> MLRNTDVRLFSTFALNPETSVAPHGPPRGLVNRYVSMGLPPWAAWCNKVNRYSLYRMSGVTQRSFLPKPPQEMDVIWLNERVRERVRTSRQVQNVYRQLKYPYVKTGIHYSDVLDHWVQVPMVEAAMFEVEKDGGFDNFILKRSGPELRSTYGERIRRHILVRQKEIQKNFVLQKQAQMLVESMEKEILPMEDGKKVEEVLEKYGIDKEQLLRDIARAAVAKKQQLASAVPQPSHVEVSTN;> MQRNLTKLSAAAFYEFVDNNFLNNKRPPVPGGSWTVEVLRNKSLADLQHIWFLLLKERNMLKSMKEHYLRHQEELGAMPAPSRLKMIDESMRNIKRVVKERDEEATARAVEIFKERLKRGIYRYPPGPPPPPGAHDKTSVVKVELSCYVEEERLRELFGRYDVFEPHKGIVRVELKLPDEVLKQKEEAEQLWTQYMAECSDVKAYHQWSTAAPSAYDYTEVELAPGIFANDAISDKGGKHSGDTETHEGVIVAARVPVPPPKEKQPPPKNPLERLKAERRSYLARTTIQLGYFPNVTLPPPRYETVEAVPRPVHPDEIEGPWEAYITYDREDGLSYAQSLGITTIGVATVLGLTEHVREPQPYAVVDPVYCEALRRERAREETLMKWPHVPEWKYEYSTYTRKHLADIVQYNYTNVVDYVDREVLLTGKSVWECPIHIDHTCGGSKTVPPHAKKPVRYMDAGIANVGVTDI;> MMRRMWVPTFSAQQQHLHHAMVLKMSTYASTPSGNGVTSAASNEEMNLHDAAAIAPGPYRRVGNIFIVHCDDHPFKHSWEVNRMLRELRLEFKGQTTIVPDIPQVRKRIWRVRHIVKVDVLDLDEAKALIGVPEHISFTDLASQLPPSFGRVKAVPSPVIRSKMNFMKLRRMRLRDVLHRDALELRLLELKRSAMKNXEQQKHAQKDERTDNKEGEKC;> MFRRTFFTPMIAQPTLLMLGNKGGTPKRKKNPMQLRRKVYGLHFKEKYLKMEEWYYCPLCAEPKKPGEWCRREDCRQIKP;> MGSEESNNICAYKRTISLAKIYIVLLVKTAMLRYSRLCFPKMGCEEITRKARRVQLQPTEYLAQHRMQVWQLRFKEMGPPFSRVWVALGGKMRRRRVGRQVDVKDMRYYWRPIEPQYQRLYMSRLRIRDHSNKLRQPMRLRATNADIGSGSSSIEWERASNRKYGAMLAPPKRQDFEFRVV;> MRSLIAMRRRFVSGTWTIAVSTQQRHRSGSGPGDKRIRTDWYRCYPSLMREKDRDMYHCYYPYLFDHGDKMSLYPKIPENPREWQPEQLQTTYDAIREDKYDAFIRLREKFPELYQDTRAWDNPPPFGEFNMFYSVRFGMVGVKAFTCKDYDELGNQFDCTAFWFPDNQVVKHSTRNGEVGTDKVYVGAMNVPVEFHKPHVAAFYKAAGVPVKHVCAGFPITPDAYAPVGTKLDVRHFKPGQEVTITFQNTDYGFRGVMFRHGFDGGYVWLGDSRWQRRPGAMGTEGQKRIYPGHRMAGQTGAAAETYQGVPVWRIDYKNSLIYLPTLLDADVGTYVRFSDTINTKGLTLWNEHRGLPAFPTFIPPEDEDLSKLATDECQLKSPPLYMYFRDEFPATQLVSQADVEDAKSAKPATAPPKKKVYDMKKYYEARKKYRQSMQKARKYKLMGLRTKAHEKQEEARRAKILKYKRMK;> MRRVSFSVVLATFGKRHSSIFSPRYDWRTSGVHDIAPRDEGDFLYQGPQHVLPGAHPLPLHHPHNTITRPVISPYIPSPQRSHPYFTAPLPELPHFSTTKPIVYTYGTMKERIIAPVFNLKNEVIYTRELDPFIFGMYPEVEELSKNLTYWMVRCQNFASKWDYETREIWRKAKKNWPNTGMGMPRVGNRKNHLYTWGGRTKPSKPWNMLMPTMDVKTWSKSNRMMLTLKMLQGRLQVVDRLTLEEPTQECYLELCRNMSWDVRHTGGGVLFMDGGSRITPSSEFDRAFFFGSFFNGRNKIVRPTVLCDEQYDYNKTAAKQRMKGPKGAKNPIPINRFNAYDAMKHDRLVITEGALMQLEDELYEHKLQILPPHIRNQLPEYGYLDSEALGDCVPSLKTIQMEAAARTEEAESDMYKSFIDNPYNPWKDNMDASYAVDGADGTVQKFVDGKKVSWSMLS;> MRRTVVQRVAPWVPPPRHDIKVTMPPPPGGEVGGRFGVSQGYSDRLARTPYWKRMALSTYKLRMMENATRYPMSEHRPGEYDIRYLPTPYPCTIRNRPLLEVGEPRQIPSIRIPVIFLVNLFDEAKGCWFGRRYETVYVERQFMREELMPQRYAIYATPEAYKLLGLPVVNHHTHEEIPKTPREYEKLLERQRYDEERWKYTIEYLFRKYEDGPPELLDRPEDGWDGSEEIALSSVAGAGRDGVVSQRXXXXXXXXXXKIKLF;> MLRACGVLQLRARPKTVCVEPGSNRLPEALVVEKARDIFGRPEFPGKRVLHNWRFFIKAGKAATGPPVGQEFSKLGLKAMDFAKVFNDRTKPHFKEDVELIVRIQVYFDKSYLFTIEPPPTAWFILRALRKKRRETGPVPLRGHYCALMTLEMAYEIAKMKPLCWGRPEYPLLETRVRRVVGQARRMGVCFIGVDTPYSSPVKDMTEQQYTEECERYRRIHMEQYTTLRQRELEEAPLIERLHRPNMSPLTDEQIEEGLRDPCLLDTLWRASHPLSPYHRDLRERELARRYLNARGWVKDMTPEEMRIVFMNYRLPEGEKRKQMDEXAMSGEVYWTRDGAQL;> MQRSTRIVMAPFKSVLRRHKHHPEGLPLYNDMSKQWLCREGERWWLLDARGEQLPRVAAVAAQYITGQHRPDFTPGMITGDHVVIVNIKDVVMVGDQWIRVPITWQTAYPGGKYRIRLTDMYERDPCMLMWWFLKDEVNRHFVRKLKTRIAPLEKAWLYEDSIHPHADKNPRPLCWTDPEVKGWKYRDPQFIRRWKPNEFMH;> MLSVSPPLRRYRLFHPRREAIPMHMCPAKTIFPLINSNNLLVKTRNSWEDFTGRKEFDEDHPLPVVGSRLNGRTTQHKWNHWDQYLNPQITQSIKDLTPTPEYVGMRCGHNMIKMGWMKIGGSWKYSRGYNDRRRVFARGQWQERKMTPRFMLAPRVSAGGPRNRYEGKLVFSPLRLSKLLWAIDTGRINPNEVITLYHLRQANVVGEREIVWPGFVLISNGVRRVPYPIHIELQNASAESIRLIEEAGGSFTCVYMTHEGLYQELHPEEYPIFMDQELPERRGLESLATNPSKRGWLTRWYEDSSKYAHPAAGRRYSHYLKPPTERDFPATVEEYEMVKHHQKWHLNQPGTGTLLPWHSYNTADLVKRAAGRL;> MLRITLLVVGRAPPVIGCTRKARYAGIDDNPTITYKPWDTTEPLMADYGWTRGKLPKFRARSPFHRQQIARRMVTEMIRKDYCIVGGARAPALRILADHVVELAKAGDTDSRQQLAYFLHDPLMVDKAFDEYPRRFKDMNAKYAMMTRLKSRRRTDAVAMYFVEYKNRDMSDNHKGEDYSAGPERFFLPPRIVETEKGIQRPPHMQMAFDRWASKFKTEEFHHWWRLRHAKLRYWGVRNVPHPSDVDPLWTEKEEEEWHNEMLANTGEYEDLDLDDESYTAAGEGGEPSPAGDGPQPQRVG;> MGYTRERTNRHFFVARANAFFSRLPIARVQRSLAMEAVREGRMRPWKYTKEQILGAPVTCNFEYNPRPVRLIGTVMDAHTEETSIKGGLKVYARNEETNMMLWIPPGNPKLRHEVTSTKGSFQHYLDERDKWDEAWITGRARMK;> MLRRTVCVQHYRAKLELDRIRSMLRGRARLERKVGLKRLFFLMRTQTRYRVEQQAHWERAIVRKNVDSAAREHGTGWQHLRNELGRQNVMLLPRSQQLLAQYEPLAFRAVVELCASRIPPPPPPVVASVPEESYTLWPPASHDNSECASTDGSDAPHGQQQSLSHPAARVELRCGVERVLRRGPSGLGNNVNELIDAWKEFDVSPLRKGEVNK;> MPSLANGLRCPDALITRTLNPLLNGPKFAVIYCGNHQYKVAVGDVIAVQRLRVEIGSHIALKKVLMVGGPRFTAIGRPLLEGVRVTAQVEEQKRMRNVVSLFATPGRRHVRWVDAPHAATIIRICEIFYSPNVVGELDKYKGELLETFTPGQHTNPVYPVDDGYDVFRKKDKEAMENATTFLDLLGGV;> MPRPAPRFAMGHMLPHRSNVGSQFLHTQRHGSRSTWYKKHYFSLRPFAIQRHHGTTPRILLDRSLWKSLWITKLQLPDINRWERVVNSRRVTEDRYAFVEEEGVMHKVNWGLYCERLETELTVTQERLPQHTLLMKAVPSSWKKLDIDISVIRGLSLREAMAQCKLSLRKGHQIVFRALEMAQQGAEAKGLDKEHLRVAHISCYPGPTDKQIDIRSKGYYAWKTKKSSHLVLTLAEDPEMVLPDRTCLPYSSLMSMKRAGLSAQPTVIDVPAITADGI;> MVVSLRRFHSYANSSRGGATTCLITGGGKGHFALTVSTRGRFYRPLVDDGINLWRRRMGRIHKGWRTWEYQHTRPDPRPFPDPPVNDYFGRSRIWNPIACKLGYVRKKADEWGWPNKPPPPTGLRYSQEFFPFFFERYFPDAEVRLLLDSVLNNETKRPVFQIPCSMSKVELVNYLKNIYGIDNVVRVEVRNRRGRRYKNEVGEIKMMDDYKVAVVELDTPVSVELKQIKGTEDTSDNRPQERITQ;> MYARFRTRSKFYFRPARPALAYNVDPNVMRRPKVKRGLLKGTYSDETVDLRDRERLELLESMRHPRERDFYQDHTYHNQWLRRDLEKHQKQQLAARYKYFAPDFEISPWIWYPGDIVEVVSGEGIGQRGTIIAVIKYKNEIVVQNINVQDVVIPASESRPEQIVQREHPISVTRVRHVDPSTNEICNIEMVKVRNKETGEMEEKRMSLESGILMSIPPVNDELEVGDPLKDTPIQDADEATYDREAEQAVLVDKRLEAMEEHFVQSLKQSYEFHEPLRRKNAEDMRQFQTDVIDMACAMLGERLLDTVNASDTSSFPAEWQEAIAMHVEEIEAEMEEVAAKEMAEAKEGGAAENEQHDDDLDDDEDELDTSEESVKHV;> MLRCSCARRRGVYHNAPSVYPFVKPFHDTPYDQDRGRHDSVGQRYRKNSWPEWMDNGADGTGYGIGLHRTHPLSRLRGNLKRSPSHVPRVLGMMIQGVWHKSGVKLYFRGGKPPNPSVHPYLTGEPCPLYGWKVTDESVIRQFNMPSIDGTNFRYKPYVALQERKIMGVQVPSDSVSLASGRTTESKPLAKRLFFWR;> MLRLCRVSLRVQSHQKKRAQHPNAGTRFGRVYNRGFIRYGFGGFGMSVYTPKKDRRFRVQPLPSLHANSLADDTPLVTTTRTLSPNFRAFALQDGGVFFTHPSHEQVMRVGQNILAEETKATGMTSMDTYVNSRIQSIIAENTVENVALSHWRRRHMWNLVRTHGKLQRHWGVSDATKGARSNIYGRPS;> MSRNGELCLKKVIISYCPSNGAPNTRQFLATHLPHFHAKYPSVSIDLRPRLWPEMAITGVYRDGSERSYNTKNLSPMGIFLRLNNLVSTANDYDQPFCASHLHFQRRSVQGTWNPWLWNYETERRRTEAPQWRRKLSEKEWDYYVGQYSAQMKQEEDEIQRRVADRTCVQEQSTREVQERWKRHVVPRMQTDLEFNLSHFKRQHARGQLQQRPVTMGEYRLFSVPDPRELGQDAVDTMRRRESHNMEVWWRKRKEQLKPP;> MLNRSRLRRVWLGGTAANTSLGRDVMPSTGKYINIVSPTDVAANISAGAMPPEANVAAALPVPRIQYSKWNRALRSDVYDELLKLPLRYKLHDFAKLCPPQRCQEEPEAVGVVGRDSAVGYLPPLGPADPLDTIPFFVHRSSNGVLPGKVFSMHPRNLMPAFYLRIQQVEGDMFRFEEELLKIFPTKKIFVRSHSIYVYNVALDGRMVLHHWLLGLGF;> MHIWRTAASNWVKRHARSNAAQWRRPEPASSSAAAKTIARLLAVGGHGCWSEATALYAEALATKSVQRYGVVTPAHRHDCIALILGAMSSSVDASGSDINRGEASLTPHYGMLAERLSLDIIVPHSDVGQEEKEAASVACIAVFRALLTSGRTHAAQRFAQQLLRSRNSREHGLWALRTIMLAVTAREEGMYRQLFLHGGLLKDLEHLTGLDAFTVVMSSCDGHEKNIGPCGGRTEGNLGRDEVHRVAARWCVDVALHMHTCPWRFCLTNEKEPRRETAFNSEVTSYCCAKELPMPAFAVTMLPFEVLRSNAVGVLRCCTAAGNGSHGNEVVTFDGTASNVSGGRSGDSTSCSTTAPSLGLPALKRLQDVVSAAIEVPLSTHEPVECLYLLLQISRDSTAPDPRRVMPSTMNILWWRRHLQSCVLESVKSAVRWKSVCDFVGLSRLVTERVPHCFPLLVAHAAESPDALRTLFNEVSRQEGAAAXPVDDIPRSCVMGLLQMCGDERSAAVIDWVVEHCXDHESIAQFVLDSLGQHQELASVVVRRLFQRSEQSXDVINALSRLLEKGTCRTLLADVCSLVPQAQQWTVALRFVSGMSAPEVGHVHTAFMAFVGNCDEQFAINMALLWSDETFTWLKADVNPPPRRVYMDDRWSDALRLVALGAERLTQRPELLGKYIRYFSKRVAVNSRLYMELEALLACSKVGGGSARNCGRSSNWNPIASTVTGGPPLETSLVGVRTEVLPKGRQWMEACAHASEVGVTRGVLEILAKRGRWEEATILLARAEAKRRVEWAPLVIRAARLSSQWRAALSVAEKIAANGMKLHYSVVAELLACCFSADVPLEVVQLWLHRRSVGESTSSHVLFGLGPGSSLRTEQRDANDKHNVFGDASRWLGSAQAELFFVLLESSSSRSSDHQWRYALQLLKEHVLLSGGVPSARVFRSTYSILHRAERWRESLQLLGLQRSVCGSPTVKCVHLVLSTLPSTAWQYALGALQCIPPGDSGSIHRVLPLLLPVSWESALGLMIDHRVMTNTAMECVVGCEDVPLALRLQAWRRLLPSLPVSMKHRAAPIYLRLAAGVADGDVGLEGTNGLDAMCVIERSIRGLRGDYINYASFVYHRALLHRHWCNDSLHPSGGVAAFRALSGIAEVDQQCEVSAAALEQLSNIVERLEQVCGTVSASTATHGSQHLERTVPVVNSGEILQGSAPTNARRDPETHCFSFVSSYWLSLFYLFRYCRCVISSSLFPFFKKDQGSGLPIFDVMRLHTVRAPIITRAAMRGYSEARSNYDGTSLPAWPAPGKKPTYPAALSELRLPQPRMRKTRTEWMYYHGHGGCPGKYGPSREIADFEYADGTPASISGRRFAFKHHQDHLLVQLIRAAATVERYDASGLLPRIPGTAEQRNWDPAIPLFLDDVDEQGRPAPLRTAGDAPGTMVSHVCSRVVDERMGTPTHTPNELANRHEGETLEANTMFATNDPSAFVSDTVKLRDDKRPYWSRRRWALTDKFLVPKSPKPKNTIKDE;> MLNPPKHYSVESLRTVGLLPAQLALSRKPRLRPHVGNLKGLVYPLPYYAMWRGNHNKYTYNKSTVCLWGEGDTRSMYHQHYAHAKCPTDYGRGGREFEYLTVKRGKMLQKPLPRVQYVAEGSKPVWLFKSWHTPLSSPSMWEREVQYAEHTPEHIGAKRPLAVVAPRTMHRYLFLMHMEKVTITVSPLLFGYGHTIQKAVLDFYRRAISARSPFPKDKVFLFYAIDHITPRIEVTWLDGTSYVPPVLEGASSQDLIQMVMEEAWLAADRMAAEGRVLNPLAIDDYKWDQLVVFKKVRDKEASKGGGRKK;> MLRHCTAHRRYRTAWRELLHPLPVRARKMEWLKRDAVEENEEILRRPYYTIKSYALPPAVGRQESIHNSNNIRGGMHSSHSLDLIMRQPRRVKTPEQLRALRDRLRFIGVTGPMPQATSVSTKSYTDTYGSRLRPRYPESWDTVPPHQPSRELL;> MLRGTRGFLAVSPGVGIAPETTPVKYTPMMLNIQNMMWWNGKRNLYRATYREKTWYEISRTGAFTKGRRPVMRQKYSREALQAALAMVPPGFEVADVPRPPQRILAQSEGIVGRWYSNYWTLHSMRYQCLLAGVEWPLGERQRPRTNYDEPFFFADFEESKAIRDYRSRWINVNRSLVGMTKRMKEAEEEARYMQFRKLQDTFWSNRKVLVNRVKSMYNQGARTSAKDMPIKTINIKAFLSE;> MLRRFALTSSVALRLRFERDSGHNTVRYRPIPESMQPKHLEDNFTPFPLPKFDESLEYGPVRLRNIPDIEAAKERRRGSRLAATEVLLQETLQEENQFATSGKGDGNMAIAITERHTEDVTTPAADSRFPSQTMSPCSHEEEMRGYVVSRDYPLIDRLHCTRSIEELVAQFEDRPQIESRVAALADMASTVSFRSDEELLRMFTAISAPFSVDGRGLNFLTVKVSKFGRPYYVPNSLLPAYVNLVDATTIALVREQPWRLSASPALFIQVLQFMALIKVFEPNKWFTFSDHAPSNRADYRHAIGVNHSTAFWGTGEELYDFMVELLRVEDDGRIPTMLDLCTREQMVDLLSGFCGVMPCGKAVGDVFKTITDAFLRRVRNDISGPWSAHDWAIVERMYLVTVLCDAGNNEILQLLLSDTASPRGPDFFAAVSRTKDTPTKKRALCLLQEAIDNASAKADKVTLLGLLESGSEFLLSLVDKGVAHTFATQNLFDYRILNSFLHCSLVADRLRVEQSVITSLIPSSLRDVQVQMLMSNERNALNPLTSSLPGNSGAIATAPKLKRPLMTMLSQLEYLNSIDSVFILHSSLMATSTDQLVSAVRRLPSGKDSLIVTMSCLRALSVKSLTSPSMKERIACARALEIVSYELEKGRAVLLPFSEEILLHDAGAYCDEDLMLWTVAAFLARELPLVKVHTLMHSNCTARTPYRFLKGGHNLLVSSRSLYDKGAPLLSSLHSKELRLVTHNVRLRTPVRDRKCTLQYYNPIRARFVYRRDKPLFDKYHVTARNLAPGFSRGALKHDWRALGVYTPDHPQVPYHPLQTWMLGETTVEAE;> MLYTRRLMTTGGSATADGAVSYSKGSYHIVPKKYTVGKRIAVRSYLDRNRTELSDRTYMPQKAWFEPYTPKKFDMEHQRISHNFYNLETKLIWTAFDTPELIGILLHDETIKGAPHLYDAEFLESAVHWTRESRYWRCIGITKPFYNKTTLRAQCWHDRGLQVGTLVFSQAMRDALMDLERAVRRKELGLEPNYVWDRWGPVGFIDGARTDHLPRFAHNPYVDPDGVEVTEVDIAPFNTHEQIKERYGAFIDPDLRPFEGVFRAPSHGALTLDDVPHQEAVRLYRDLMEKADMPVMLGNGAEIPPMDMRALFHLSANPERMKAASELSSWREVRGMLAPVQEVCDEKVEALRLMENTRHDAARVRTFYEEKCGFSDFMRTPDKVITAAVLCYLQELQRICTETDWGKPLARCLTDLERVNVMGKDAFLVYRHIEDAILDKKRRVWATRFAGEANEESTLDYLLENFGRRTEQTRNVGTTGTEFDREQEPIGRQVQRRVLDSDKASKLAEVRQKRGKMWSNKKSVFDSLHQKQLQNVTYGVH;> MCLKRKAPHLFCFCLWSIFLSFRCFCFRSYAIMLPLLSFPTIQISIFLSFKLPITTFLLSPCFVFVFVFAIRYCGELTLNAQLVLFLLYHCAQTQRGPLKEGEMPICPGLCGELAAVPFRVFLGTLPTLAVEERFLRQLQPVFAWYSSRKRVKEQANEFIEIDLASCDAELLLRYSHIYYVRRQLFDELIERQMTLLDSGKAPKMAEPSLLQCLAGCNMTIADRLQLEIRQLGAAKRAASVPGRRELDPVARLEVYDYACMMRLVEEDAGAVGDAEMKARAYLPREVIESKLGHLTQLLLGSDARAALDKKDVKLLNRMIPPDYTRVGCVEKLRPFDVTAYFRFYGERINNVKVENYFKRALWGHVYRRFATTPSFLSGVSTYWARHSGLDASFTTTTMPQEVAVAVCDQQIQFPAIKFRAQYVYTSPETARQLWRTDAAVPLMRLFPLMGSRTAEDLAAGVLTDAFWMHLGLSEEENLLQDSLLLKVRRFVDEVGDMYETNIDSVLKRVDDNFKQVVPQLKAEDLQVDAPLQDGEGEDTVRETVAA;> MLFRSVSCKNYQRGGWSPGSKHQKHMTLNPTLYLYRFPGPHGPGPYTMKYWWTLGCFPTGMEVPFRLHEFLSTYQQEHVPVEVEEWLRCYIKDPLSELVNASNDFFKAVEVYPEVESARGYKTLQPSIAPLLVPMKKFEEQLGVKISPVGLRSVLSNPVLKDRFLDDLFDYKSYVEKGGSTPHRRLARSRFEGSLSVLGECEKCLPEQHQVEISESLGTFIGATVSPAETTADDERSLILLLTTISEGCINAGNYSDAASVLADALMFCHDPDSQATTHANISFASLLNADFKGAEYNGREAALLQPQVKPTSTACARGYVGWAAAAAYQDDFEKAEAIVKDGLTLYVGNEHLEKLANKLQALREEQPSVYKQVPRSLRESRSHLPSQQSRGLLSGSGKGFSNEFDWVEFKNKLYPSKMDPRNNEMGSVFRRVGDLGSFISTSRSMERL;> MSRSAFSSRGALLFSSAPLQCQRRWVTRLYTSYYTGVLYPNQLVQPKQRLPADVSVSAILQKRSEPEAAAERGSNKGDKVDVSKGEKTPRVSWDDADSTDVMRVDNTQQLKEAPQVERPYVPLGEVAKLELQGDYYMEGGMFQEALEHYGVVAKAYNYAYPENHAQRIGIRIKLSAAFRQTGRLESSLANIEEVLRMLDASTRPSLELICEALLELGITREALGMKREATEAYEEALEVVNSFHNWGESHRMLRLLPRLGRRFNYNFEEKFVYFSPFDYDRTFALVDQCLERAETIFNEIGDVEGAIRVLQQRKEMIDKKFFNMRDFAGRIHTMRGHWKRRAQHLTNAPTPDELLRYSPTIHQVHRDFKYELTAPIGREKEVMPGVNRLVLDMGNPYRRRGRLSNKMLKDADHKFANYVRQKEYNE;> MLVPGLSLTRRAVTSSCCRPLHVVRGFSTTCTLFGLEQLQDVPTSTSRRPTGLHRGPGKRQTSEREAAQYKFIRRWELQMRDEWDQLEPFKGLPKPKRQFGNEAAEVIWPYALLLERVVKVHPFTKSIYVYYAQRQSTARGKLAAEIARSFAREFLIPITFHNSQVYTEAEMLLEYSETPWVVLHSLDNGQKPRILPVAPVEGTPAHTAVEQLLAEVVQGCEALGASVADPVTATRVLNERPLQNQYVRVDYQWFGDTPDERASHLVRWEFEPEQIEPKIRHRTRHVLDWLNYDGNLPTHRAVHVNAMREKARQKAPRTVAGPRTFYNSAGSRANARSSRFGGQAAVGK;> MLRRSDLLLKKGWTHNPGRTRRGGKNLAWRPKMSERTLEQFVPLHLAFPRRHPNSWQERQFHLLGYVKWPKEIGFYNAGDNFELTPQAAYRIYKQNCDETFWTRLHNEKTIIHLLPLVEQDPGTNMVLVDDIFRHHLKRFGADHYIYNAVMQAAAFAKDFPRCEQLLAEMRGLGLEPNAQSYVNMMLGARLTGKPRDQAEAFFREGIKTGAISAVMRLDTEFQMWMNQLERLGSFKAKVGYLSVNEEGASPMPRDMWALWGWHRTEAKFISRKQMISEQVQNRVRSGKELVGTVYQKARRQPWAKYNGMFPYDYNGPARRPAASFVDAPTPTHNAEVCGTAY;> MLRLSSWNLKSQHHNVLRRSRPHIHKYRELNRWQRQAQGISKWDQSHSHRPLPYVERFNPESVGLTRGTSAFAWKWWHTQYPWLPNVPPEAAQIDEAQKQERRSHRPPAWDDEFAKVVLNMNDAEIREYLMSKLTDVIFLETQRDGYELRRLDFEGKPLTSLPEPRIIENFVLEEETIRERVIYQVVEGVFRLSPTSADRRELRSVANIIDYVLTHVRAARPTDRERRQERPITSAALAVMQKCPIQPQLGFVHALPHDTRDALLQEWERMHHLDWQFGKAVYTPRSKENVRGNLTWLREDRHYDQRMKFMQEVESGEARAKHMKLIAEAAGN;> MYVFRFHISSFHSFLVNFLQPSRGVGEPSRLLXHLETHPSYMRRVTSTAVHRTVSSVLSXALLPSFNGTLLLSVCFASCSAAPVRNLYKRLGLDHKATSEEVKAAYRQRALECHPDVVDDNQKAQAEVDFRAVSEAYDVLIDPQKRKEHDKALGLERTVPPAKKQQEGEGVGCDSKGSFNRGVTRPRNRKPFVRGDADRNFREAFHGMSLDQVLFRERLRQRRMQKQMEEKAKEGDDGSPAGREESIRRVAAAAAERFAEKVRRQYGPGMLRHARVYTSLSRDPQPPPSDYMPFRPFHGWTVPNGVRTPPEPTLGPTAKVEDVKDVQLAEPAVGDASHQRKLPKHFPVVQASDGSSLLREETIACMERERRLPHNMGKLYSYHRPY;> MGASAGLIRRGGGVFPDAVSLTLTPSRRVYGGSGRGDLLYENPDARRHSGRALGVLNGVRHSSQATMPESGQLYYRKLILHSRPPNGSCAGLQRHCHDTCNWSYLIPSLHRCAESAISAKLWEKMCQLGLEDRSKAWVNLTQYERQRVRDGQNLYRYEVHQRLPLLEESIGWAQLDDLLGWFRSARRAWVRLPTSVTLSRESSEAGVASVVSPSSAMSCRLEGHADSRDTTPGRNQVFDTPERVEQLTEATVHRIREELQRLNRSERSDCEGSAAMRASARRLARDEELSRCVEEELGWHGVALQHRIPVPK;> MCCLYTSDVFFWSSLVVSPLPRIVRCVSAPQIRSIPCGSGDFSVMKRSLIARWQSGVHTPHGVVYRGAKMKNWPEQRIPENFKFTEEQRFRTKAIPRDVGTIPRNFVLGVLYRHQPCEVGGLWEHCTNDPEIVLDSKRHLREVLKQAREEGFVTFERDAISNEWLCFLTRERYEEVQRIVTAKSEAVDTHSGLRGAAATETSTYAEKFREMNVEAKEAHARRLEEEVANTTRYLRRFQQREIDYLPYTDLNGKVNFMWWYETRDVQQRADEVLTDSSSSKALAGEEEHKAGSQLEATTASTS;> MKRLFPSAGVSVVLTSSSIVMSCPCNHIFTSRRAYYWPYNEDFVPEGAETSRFQSSGSPGTRRRVLQEYALSPLFGARVPCCVVGTLRTAKEIIVLKRDIQSLLCELMELPQGSVTLGPLQQLREMMLYRHGTPLSPRLGDERQLNMDAYARRPIAARTMMDVFLAEDMSLDEIVNFGRLSLGKLQIALNNLRKENAEKSSADCEDGSAVEPAQLLVDRMGISYCEIPSLDESDYVFAEVGGVAVTDEEAERVAQRWAERCE;> MLHRTRLAQLINGRILQYFVPYERDEVNPVVFMDVTVEGDALGRVSVELFHDIVPKTTENFRSLCTGERGYSQCPLFYKGIPFHRVIPGFIVQGGDILLKDGRGNVSVFGFPFPDESFEGKAGKHLRGTVAMAHSAPNQNGSQFFFNLARNDHLDGKFVVCGQVIDGWEVVDRVAVLSGSSCGTPVSRAWITECGQSSGDKLEDTERALSGERALHTMPGKEVLDILSPRY;> MLRFTRLFREMAPELQLEYMPVLFTRTILGPQGGFAGEERLVKLEVARKYMEAGHAVTPTEELRRGLWCYNPDTDKYDCFIERNEEFLDFAARKRQWLDVYWRVNTGYLLFGRQSWGQGFLINCPLRKRDVAQKLWEQYKVRIDPRLIEFREKDRRTGIQELGHNWCWLYLPGAEELGINREVYDNKRVKVRIHVRKMNSMFALY;> MRRLGVFCRGQRNSPLLTRGIATGGRVTNEDRRWWLVHLECAPDITPGTFIAWLDCCGTHTCKKLIERNIWTIEQVAALDSDQVDELKYREGCLKMDVVWEHARTIITPLRQREVTGGVESELQGRIMELRKKRELERRREEILKERANVSEQREETLRKLREAIAAKKAAMXQKKQAASEAYGGSSDGGARKEGAEE;> MRRCIPARGGFTMKYKKGTGLWDEDHVNDYKTNRYLSARATMRWYQEMERHQTRNSLNARRATQSHNNNRGLHHTGRGAFERELERRGVQVEKYPLTTTTGTMRVAELVILRRMELEKRAEEALAEQRGELQKKNPTPSEWYDESKGPLNPNFLRSMRSHYEVDIANLPDTPLIRGQREFFIGEERGNGAA;> MLNPTFSLYRKTLQSYPVPPKIRHYDRRWSGSRTNPYNRQYWRVIMNENYSRPSFWVSDFRHRYLMRTGTDYQGQVPSSPQPGLYQGFSDVHKLLANHPKPQRESRHLPVLPMTPRIVFEHANEKRIDTAKRMRRDRRRIEELKTLEFWGWYMKLQRVRGRWCREQGVSSRGVYGPAVDAAELWG;> MLQINAFKLVRATPFLLKRTGKPADTPDYKQVYLPYDAAPTERELERERRRFKQAYHGRMEHRKLVEVKEVPLNVYTYGKEGMSLPIAIFKDQKDPVIGPEWTYPGIYENKIAAQHWYTEELFDKESKEAFESPWQQQILDNQVKRRMAKVMFRMRQVNMKAVDLFQKERGSSRRSGGAGEKGKDGGGKK;> MSGAFGCGSYRSVVAGTQNVPRRMTFYPSAYELIQLHKAHREVIRHFYVRDKIFDNKFPGNALANGLFKFVPNRRENYHMRELMESIRRRSIWMHRIKQQREINAKVVENMEVKYGKKAAASMLCFTTPDSNAYFAPHRYQDVANSWPNYWQHPSVNHVVPKPRWRRHRELGGITRVEDPFAVQASDY;> MRISERAFMDIAIGTKAPRRIVFKLFPRKCPSAVKNFIELCSGNVSTDTYESGNRDKLISESALPQLTYKNSTFHRVEKGYLIQGGDIVTGRGTEQLSIYGGTFSAPEEVRASVFDKPGLVGTASSSPNAHGSQFFILTAKEANHLNGTCICFGQVADGLDVVQEIEQVPIDPSGFPSLKVSIVDCGVLE;> MFRVTGLQLKNPVVFKQGQGMFSHQLKRLLQKKSIHRYNWDPLPMYDPRKLVHASRHMDVETWREVPDPHWDERSYLVPDQMFYNIPVPPEYKDAYWWRELQARRVQCPVEWVSHRMYNKGDRQRYDFQDLAFRKKFEFSYEEVVKNAKDMRS;> MAQWVPKTAWKVSNLNKRYGPGYITSGFSSENTLGYTHMVHDSHKLREKLSSRKGIFVIDVRDPGERKLNPVPRSVALHHHDLLSGASCPILPQQKSAAELFVLASNESRGLNSAAALRRWGYDSVVQVDYNTLVEAGYVSRCDYATAGTKDSAEQAVSGED;> MFRPTTAIADSFKEHYHRVHLPRRLALQRYARQQSLRNAAKGNVKAEEVPYKYNRWWVNEEHEFVHQYAFVEDPEVTKAKRETLPPVTRENIWKEPQQTFFLPFAPYVRVVDYPKDPDAKFLKPVNIPRWKDYMQRTKPVIPRTWY;> MVLRGVRLRSVAVSCYGSSLTAATRCLSVRTEDFFSKEAISHARRVSWAPHTTEKKQGAFAKLARSNFGDPLPSSFAQEPYFEEEIEAHRKHHRPDVYIYKYNVSPTHFSLRE;> MWHSSLRYVSFKRLPFGRRSTSGGVNFNKGLLTDRERGDPFTEPHAYRNKKSIAAISKVAKKQDILLREEKQRKELDKIQSGYVTERELHIGCDKPLGGNANEIARVIDEQALISPTPGEKCSTALRELMENEVDRRNHMMDKFGQPVGAREFHRLFKELRHADNEAETIERHQTRLVEEYGVYPSLRLDAYMLDDDTYFPEWVNALPYSIRDRVKFGSLGLTEKDEALRVTLGRMPLDRRRREWERLKKAKEYKAAKEETLTLAELRDARQGKRRFHWLQRKRQKRASILRRLALRKPDAFELWPSRVVDYSQRIAFIAQHVENGLDTKGQWPLDPEELARARVRRSKEEAERTFLMSAEEKRAHKKLSGRSGDGSISEMLQSLEVPDKPFKRLSRKVYANRVNAIVHGDQDEYGRRYRKMETRSKRRMRPYASLGEIGLENELRKEPRINAKGLNNTDDEDWPRHTKSWGDGMPSMRYGS;> MYVKLQTRSIPSLFLPCHINFDCVVCGGEGEQAQGKKDTDAHILVVCVLQQYSVVTNSRRGNRSSCSRIMLRSFRSNAFGLLIPGACTIRGRHLPVSSLEVTVGFTRLTSARALFSATHLLWRRQHGPTNVLFQLDALPPNLQREFHKDENAVNLTYLVDLPSSKIASSHEDSSDGTTKSDTKSPVIKVLPTWAHIVTWCCATCGCQWSARPVDRTDPQVAAFYSCPRCAARTAKTYCSDTPLAVSPSTPSFPPGRRFAEAFPLLAAQWDACRNSVIHNKVLFESVADVPLPCATIAWWSCPHCGEPWRESVNSRVQRLVQQQQKHSSNGNVRSNNTCIPLCPSCEDRGLSLTVPKDGNEGSKEKSSSERRSKKKGNQNSELKRFLKDSPLLLAEAQLQPHEDPGTIALRSNKLVCWKCRRCTYEFVASVADRFLRYKRCPQCTGEKRTPLNLLSIQRPDVLREIARTVVRGKLLKMTVHDDTVVPFVCRSCLSIYRMPIRLRCLLPEGTTACSKCMWSRSKFTREVVSVGKGQKGAPFRSPPKKKRGRDSYAVVDNELHLRDTDLMN;> MMHLSLQLCKPKTLAHMFRKLKLAGAHPDVLWAVDAQKAQHNSEEMIRLETMMHQRSTPGASNNRQSTAESFTFWLTDNQQQPRAFAAGRSSLRSVSCTINPIAPTRTIKQQLTQLFRDAGVYEDFEIGGEGVEMNLESVLLQADERQEEHLQQSGTLYIRGDKSIEMLRRFGVLLIIEEEGVTYLVTLPDVLDKPVDDTPSTYTPARSLIGPDGEIDPRVQDYIRDRGLRAFDLRMAGSHSSVERFVSAFERLERLYEVHRGRAMRSCVCLVLSIKAPKCYVAEDGCIVLSVQQMPMWEEFLLSLPQEVWQSCVQMHRDWRVGNAPKFHEQQRQLMKVADMFHFFRVRLDGCIGSQTDWQQQFILSMQKEEMIVRNAVKKYNLKSELLKRRGEICVSNTLRSAVDPTKEIGYRIGGDGRVYFNHSAMNTGQMLRALKDNLRRLETFQKQHDDAVATLEHMSRSIPVDFSVDTNWKLREEGNLVSCLQRFVRTIKANQTQLSAFLTMLLKKRDGAGAPKKRMVWIISERFDTLPSGVVYIPWDVDFDSIKKHLLPSG;> MWSKVFTPLLTHRLTPAEKFPQLQLRVGQQRRVTCGRQLSIPLSSFDSHSLDFARREIEPGSVVELRDADHRKLLALAFYEPALLRVDIFHHTPKVVTDLPRISEDFFVNRVKEAWGRRQSVFRHVRTGSTNAYRVVNGYADGVPSLYVDLFSSSFARVVATSAGAERIVPAVTELLRQHGVEEVLLDTPHLKDHEKLTLITPTITLPETYMENGASNMWLPRDEYPTTSSNRWLINTAHRRIRAVLRDLCHGKRVLCVNDRGGAAALQAVMTAKSVVFAESDESLLNRVRENLVANHASAVFNTCETTNSPIEELSMRQQDVVFLEHRFDTLSSPEQWQNLLKVMLFRGVCGKGSIVVVAQEVALLGMHDYVASGGGVAASVVRATRSEMFNVFNRVTAEHGLRARLLRFFGPSIDYPTLPAVEAGCYSYAFLLELAS;> MRPLRCSFGRRHRVTSAAFGVSQFPSSSSTFSASCRWVVIPPVEPITSASASASSSSSSSRKGECRTSYRFAVKDEERGLYDHGVTPDARTLAAEAEAQYRASSEFLHAPAGGLPAPELHMEVDGTSVSCIAAPFGEEYVPSSKERFAHRGHVGDLSRQRTSDRKYLLDARSHLNIRKERQLSELLSAPMPLLQKSNEIQQMLLSDFYPQNLVVSSRNVEAVIALWAQCSLEQCIAGLNSQRPENLLAPSADTTCHEVDAVDSVPFLNHMKRLYFHSRQTHVAPTPLVLEYVMTALGNVTTADSRVFHLANRLLLDADKYVILPTRTTYAAFFTICSLHNAMPFALSRFKDAVVNLHVAVDSTMASAILEGLVQNGLVEEAVLLLARLQHVPMDVQLLNTALEVLLLSKQPQSCFSAFEAVRHSGVEPTADTYTLLLLACERSGLWGNTTAILADMQMRRVKGDGRTLNLLLKGLLTERLHGYSRQLYETMVNKNVEVWPALESHMKSRTAGGEQLKRGSTIKTSKSSQPS;> MKRFIQSRRVWNLMDIRRRPPVLNRLRGVLQFAQQPGALSRHRQGGDYNCSMRVSIYSRPGKVSRLNNADATWHNRSRKEKPPDFDPSAFRRRYRDS;> MEKRARLLLGVRMNYAPFSFMRRRRITAAALPVAERSDPLSICYRCVHERPFVEPPPEGDNNSDGEAYETARDALLQLNMMVRRGIEPDALMYTSLIATMGRARLEWQAYKLFSRMLESGIRPLPETYVALHDATSPRRHHLRCDLQQKIEESLETFPEELAEAELQLQRERDRLCVQKFEEYMSGVLPPAPPPPPSEQEAISVRDKKREGDRSSSFGGGSNAAGLGKSDAKPIATMHIRNPTDAWSTAQMMDEQQKLGNQRAQGSTAISLCEQLDKLHEEELRIFLSAQRQLRHGNKTDLVKRVLHCVSEKSIRDMLERRKHYFQSVAHILENDLNSLRRDGIIAENKADESVNNEGTDAIPSAANSGGSQPVIISYACGVDQTITAEEKESVAPDFLHTPWGILRKPVRHTSTGEKSRSIDRLQRLSLNVDELQLVRSKASTGDLDELPESLLRRYAYQFSLTWKRRHPLSLLEAVQWHSTTLLPQQLNEEGGASPTPALRRQQEDEGVHKTLENYEAFRIISQRTNNLQVVDNKEINLHLKAIRREALRKERRAEETLRREHSLLEAAALAASAKSFTPPEEDMVPSSRVLGVDAEHNNDNESSGRLLPTSSDWEKGESQEDEPKEXPPWAIFNGEEEFNMTTGRFGDPRIGRYQELSDGRFKILPSREAQSRWTVNRQLLPGALQDTLQRAELQQKTRVEAVEKVHQEKLKFKRYRKWDAFLRKAQDKQKGKPQTDDKEGDGDGKKSAGPLPAKKRLSLLLRKGKDKAPIDDAVKAKYCKTL;> MPRHLSSSLLQKSLTPGAARLLPQNLIPQRRPAPGRMTYRGPLLAELDRVRDTCTTEATSSGVVEESMVSNGAFDAVRPAALGSTSSVADEYLVPTPRATKLKKAAMAASRTPTFVLPNSRSATDGEGGARQANDERDGTNSSPQLFSIESYETQQRALRNIFNEAGRHCVRLRKDSKWLLEERRAFRQSHQRAPTTKEVSPHVDVALAPVGALKLSKYLSPCSASREVVEHSLLLHRTVTKSKLVQSSEKTLFRCLRCFHVYAARPRTLLRGEVAQSWLEYEAEAEKEERARQLARRPHLRKKKYSIGRQRASLANDPRCCPLCRSTKAQWMMEYVHHHTHG;> MRRCIPASVLRXVLLLQTRLVSTNTQTPPSGCATKIQNESPMNGSFNLPRERQILGGLHADWRTQMKRSGSILNDITPALPDTKRTEEQRRRVAGWRPVVKLLGDQRLRIAIVGRMNSGKSSLFNLLRLEPTVPGRSNVVRDFDGITRDSVEGQAQLEGMHFTIIDTPGMVQGRMVEEAFRTVETADAAIFVTAVDEDIMPEELSLMQYLHLKHMPVVLLANKMDLIQEEEEEAVLDRYNSLGFGNAIPFSARRKSGLEMLAAVLEPLYHIHAMHKVENDWDIEDLAMQGDESAMEEIRERNCSDRFIRIAIVGRTNSGKSSLVNRLVGFERNRAVDEKNSTRDPVELPCSYKGRKLKLIDTAGLARHRYRADRDFIGRIHGLSVNEIRFAHVVIVVFDATEGHPNKYDMAVLHSVAAEGRPFLLCANKWDAVLDQSATAEAIDFKIKRQVREVKYSNAVVVSAHTGLNLTLLMDQALELYDKWNKRVRRAELTRLWRKMEKSVIIPYHVARIGRITQVNTRPPTFLLQLQTKNDSNTLPKALQEMMKNTLVEEFDFRGVPIRLIQEVKDSNPDYI;> MGRRNIVLLHPTAHWTRARRSFVRSVALTTLLNCSGALLTTSRGIIVPQQLKAYGGTFSRSVGERSNHLVSDVVLQSLSPSSTHNSPLLSKNIKTKTVTSFEDMPLYPELRSALRQLRITTPSPIQQSAVEVIMQRKDTVVAAPHGEGKTLAYLLPLYQNMIKDRDVYKIPLRERRPRMILLAPTRELIAQLHHVCSVLGEATGLHAISFTSRKRANHRLSRLLKQQLVDVMIMDPKIVLRLIRARRVFLDDLRYVAVDEADGMLSSQHDHDAVHLLMKVQKRVMFKHLWPVQTQTVFATAFITRKLEFVVGKKYPDAVTCIRRQRMHRPPGTLRHRFLPVEREREKMDTLQHLLKKHGNRPREILTDIEEEQAYSKPHYLSGSLEELVELRGLHLRRRPRMERHDHEGETPIATLSSTSAGDVSNYKVEENRSGFAAKGDNADEMKERVRHALEGVRPVHWEHLTTVAAPFTCHVPRTVFADGKRCIIFTRGIDCATAVYHRLRGCGYTCSLLHAALPAAVRRRMFADFASGRTNILCSTDVAARGLDLHVDFVVNFDMPTNALTYLSRAGRTARQGRLGQVYSLYTKRQGVIVSAVRAFLQKQLPLEGISNWKRHMMEPRYAEWRTHKLNAIARSYVSLITQKTIPAHLERTYLRHNATWRPLFHPQTTGVHGGVPPRQQQRVMDAITWKAVCFRRGLLARRKGGRAKFGTRAAESGVWNDVGGITSRVVANMEQNPHPGGDDFGPPRGPPK;> MLHAVRLLSCWRPAAIQHLPDVAPXAPVQEVEKSHARYRPLSLRARQTLSEKSDDLQYHVVTQEWFGERVDSFLTCHYPQWDYETIKRLVQQGHIYRYRKNGKKKFTRLTDRLEFDELLVVPTRAFWEKQLAPPSGVLEETDGPKFKLSATAREMAHNMVLFKNEHVIVINKPHGLPMMPTDDPQEMSIAAMLPAWKFTNVAKPVVCHNLDRETSGCVVLARTRNAHRMLGRMFVKRVVPNSVYWSFCVGKPTVNYGRVRMHFDITRGNKGDIIVARPSPTKTSKVAIAEFVVNASALEFGSFISFYPLTTRRHQERIMAAHALRCPVLGDAKYGGDAAFPSSLSLFWDPENKGLPLHLHHRKIQLPYKNTAGEFICVTAPLPTQMEKTFKKLGWPCEVDDPLIPG;> MKVSSRGPIVRWALSRPTSGLVSSPSEWRCGRDLSDEEKHSGLLLRIRDICQPLAKNDQLPVAVVKAQPSDLQVNEVDAVGDVAALSKVVKGKWRKISRQKTLLIEDDARTPFSDPSKSFSPRVQSYGEYVRLTGKLPRDLPVLRFVLYRDSYSLNSVENRLGYVLSLQPDCVFLRDQPGGSFGCITQHGVCLGVTKEILSHASRHYNLHPLIFEPREYFSTDKLHSLLQGARGHHHRVLLRCVEGSQDTIRALLKKTAERGFINYFWLDRFSVGTNRFFDMAVLAARGDYLKSIGALLHCVAESNGVHYDHFLKYLNADPSTVPGIAQTWATTAKHMRSPNWIVQLLRGLHKYHADAECGKSSYLAELWSALPMREALRRSAAEFVWNAMASQRLLSKGLNVVEGDVVRMGPADSVSGCDSSSLPNNCGNYHLVTKDDEEKGTFKITDVVLPVPYGSVAANNCLFPHLSPLDKKLYVEFATKHGMSFLFDEQMPSPLSNPLQFYRHLITKPVNMQVSVIRDPNSLTSIKSDLAVMQERKLVQIGDIDYSTRVREPCVYNVSERFTEKMEEILKTHRGPNSVVLSCYLPEDSSPFVMLREVFDLRHASFHDLYGLL;> MHWPHGKCGIVLTVRLPLLVVDAMPRRNFLRAPLSHSFMHIGFAIMSQRRWQSTIGEQRPTARRSKNAYSHPLAPKDPASRNIVVPDAVHAKVGSPDTLPAEILQKRAQRALLMQLQQNVIWEGTVISDERHHLIQHFVKLRQNPKYRSSKQMMVVGGRHLLHELHKRGYTPRHLLVREGQQKPKWATNTGVKTEIIRVDRHVADVCSPGNDGFIGDFDIPKPPPKESLIANKQRFDRVLVLDNVDDPGLLGTVLRTAAGFHYDAVIATNHCADLYDHRVIRAARGAHFQKAVPIYTLKEEDGDNVYGMLNHILQRNDLSPVCFAARDDNDATDELDDLVRQLRSGCAQPKSRTSPCGSPAVKRETLSDYCRNNFTKSDAKGQLLMVGPNHKRNSVRRWSKQLSIPVTQLLLDEVSQTDALIAFSVVLHALRPHGNWDYLPLHNNQEQQETASLELQGMKASVDIGPNRFDLNEKDLSLDEEEQVEKARLDNELMRWRRLQRAQGSDYDHWMEAETRRIQEMASNESRKQVSPWARLRTRWQKGAVGMPPWVPNIVDEYRTPLDRDALRVEREVSESHVRPENYDR;> MNTVKVLLRKRVVRAGAFEDTALALTNARSAGAEAKGRPIVLQSLDEVAQVTPTISFSGRQLWNSTKLLRENGNVRRSHGACVVGGASAIRRVWRDYKIRPNVVYVPDTEPTVASWCLEDELPTCIVRCSPVEINRGLLSAELADGHAAEFPIPASPSVETFLGEGKPSRLTSMLVLVGLRIPSNVGTLIRAAVEMGFESVLLINCLDPFGEKALRASEGTVFSPQFKIFEPGSDPVSALNSIAVEHNLLPLLALPSQKAETAFEVAKNLHKINAMRRSQEAEGDAAASHNHIGPLLILGSEAKGLRDLAGEWSVPRKFVSVPLPNSTVESLNVSVAGSILIHAFRPAAEKHFVELEESARPRTLGDGPVLLR;> MPNIKGGVGSFLMRRAAPKSIRQKYQTGPQFYKRKFFQFQKGHHRLHRRISGVQTGSPTHQREYERFHHLPGDVRTRPQFDFTFGETRADRVMFAWRKRGDLQLYQMSGRGETFVCYRCGYPVRSQLVAVKADNWDYRMCYRCYTNTVHRGMENDT;> MKSVFDIARSHVTFPVSRDGTALRRVLKDWLDYTECQSLQAKPAFPAELCITVHPSVKSMSRVYTQGDPKMSGEVCRRPGEAASLSYTKRVRLLLWSAVLPWEVQRGLSMSVLEPPGNGGSVLGEVGVRHGLGGSGGAVDGGSAVATKGWKEVEDSLGVVTDPTTXTAADFVSGPQCSTLGASIIPGMLFVMSPESAAQGLCFWSGAIRQPIDIAFIAPVEPPAADTPSFSELRQRRLQLSLEGYDISRFFPDGELESPTVTFAVQSHSYLDPFPDCEQRDQQVGCGSSRERNKGIEDSRRYTATPEGVGRGNENVRYVLETRRNLLRDSIRSALRECRCTHGGVVWASNTGCAADGNPTGTGECDVEVTISLTLSDELKEDLREKARLYTNYVVPLEGHVRRHIKCLSGISPHPKGDATDGSDALQQKGTEAVWGEEGCVCTNGSAPFVAPPPIIKPPLPVKVGTLASTRPRSPMLADEAEGRPTRLAPSVFGRHDAPALQRAQQECNQLISASALARIPNTSPRAPEIPPIDYEIFDLCLRLGLCQSEAIYYFYGRIMREWSKELRRLRAAKSHGEGGVNDGNDMVLREEDVHRMLRLVHDPSLQVPPELSACVEAVASLRKITNEVGVPVV;> MRRLFITTASTLCHSLHCTDTRTGGAGKESTPTEVQCEMTLQCSDESGCSPFLSSLLSPVETVPLHDVTRTYSTMDVVDPPARYNPMVPNVEPSSSSAGHMEQXLENEEEEGPVACAHKNGKLWGVFEGSEDNKPPAWFYRLCKDLFYRTNSEDNMDDAALVSDIEPSHYISSTENRHVDGSDTTQRSAEAGTDVSDGVDPYVWIPFNLLDEADYHVGPYRFPSTATYTHEQRTLLCLGDTRREYVHFCDSYAFPGRAQIPTSVGTCPSKLYVNPKQQQPVVYIQLSNDIPPAMWLPVKGTAASVRRVLAEFASMAALHRDWHHDEFMERHATAVRMLELQRLPAGEGDILRYMAYDARNAQFAFAPIREFPNQQEFFLGEHDDPEKLMEHVDLCPLLFAIPHMRTVVDLHAEHMIPTIAGPGVATSLYRCIYSKALLFVQVHLSSEVKLPPQDPEAFKFMWKDSQVLPKMRIPVFVRVVWPTNERMSGGGGLLRRFNRLFGTEFASDIPVDAAMALLYVMQWSGHIKDFLGVRGMRQRLADLLLASQQPEPTKLYPGTREIPNPEYTVAERLGMHVQYLAQLHDPDISLTIQRLLPVASAPVRMGCAKAALIAGDRELFRHIVSSEPPGRMQTYMTKLVRKRKTRDLVDAEPRLLEDQYEFAAPLWTKRGKRLDSNTLEGVVEAQSRLSG;> MRRGLTCRNVHDPVFMRNVKRVLASYKESMDHSSRKGMSREAFVDINEKGAAWYLGHMQLASRTLAEKVKDADFVLEIRDARLPFTTGNPNLQKIIIDRPRLIVFNKAEMSNEDCNRVIQQYYERTGNFALFTSAKRSWRDTVEAVQRFVTHILPAQRFKTTANVGLVVGMPNVGKSTLINSLRLAHEYQFHREDFRRPRTPEAVSIAPGTTRGVKLVPVCKDPNIVLYDSPGLTLPGCFAKEAGLKLAACGIIPTNDITLPRSLVARYIYDVLSAAGVGEHMAECLHLPRAPISFDDCISMICERSGTSGQTDLGNLDPSRAQKFLIHDFQLGNLGRITLDKLPNKVRQAVSGKEYQRIGGGAGSGTEASNEENEVVWTHDVKSSDVVARYSEEMREVMEELQGEXVENTPSNRKPCGDSTVISRKKGPISRVSAHDESFRRSIRIIPGR;> MRRCGNDRAVALLRATTEAMRLVKLKLSPDRTRNEEIQDRQNAFVWSDEHIFRPHQHFTHDPCSWSRSLEQSMKKQRKLSMVERLRSLEQRQLEEKQSASATAGGSSKCANHMDGEKAEGPRFYGAVGDSEDLKEYVANEDYFYTMQQEEKPNDPPLQELVDEVQSLHVLLSSPRYEDTPLATVERLQCAYSEALRCVFDRVRNASVGKTMSCNALLFSWSLLLQGVPALLESLAEKRTEECLVRALSTVHEALNIVLQEFNRITHSKERVELLPLEGWIESLDVVTHPLTNKDYTSLKGNIRLPESSFKPQCKLDSATVEFVHSRAIQAAAIRMIENDQSDVETEPLDPYHLYILLRCMVRLAEKGVNDSHIHRAALLTGMVGERIFSSLERTVAPPRRYSLRHALLGKQLRDASKPHAIPLDVCAPPGGVKKPPTAADDVLLLTRACTLLMKVATNVLPQTKFKVLETVDTVLKTLSYAPNYDLSTADTVIFSNMVLEELHHVDEASATDRHLRVLLLLSRLRLSMCADRSALSHLFSCLCNLLPPHSIQQDKLREWKRLRGLVMRHLLYSVRGEEVEQHYTRVLKSSETWVEHLAFGQYSGGLPLSLWLEACHIYLTAGRKLTVSCAEALITLRGRCKDGGVLRSSNSAGVGPLDFVSVTLLAQLLEVVSHGCCSADDLVASPVAWDKVRQTIQGAIGEDENTIQLLRAGRLCVADRQATGSLVTTYP;>MFTVSCNVAFLCHPAVHHSLLLLRALRQRHTLAIERMGANVTNIGGTVSLSQCGNHISIVPPNLHGSKCVTSGGSIGTVGESPLCVAEHGLQRVHDPQHILYLFSSASPVRQSALDGQIQSYLNAVVVSNQVLRAADDVLIALSIGEMEAVRQTHGNLIDCVAALDASLQQTTENEEGGGGNGATQEVDCLSTWPLFTTIQFLVEEGGLPLGPFPRMSRAYYRLKESTPVVAHSQLVWRTFELSRGPEGPTGELPAWPHRGFLRDIQRQIAEYTTDPPERIMAGVTGEKGPLRARVSGARLGLQRTPARIPWTMQGLHR[2x];> MQRSQLARKFATQVGAYSLLRGRCHAVSTWKVMATQAVTIPMYLPVRFHSEGHAAGEEAGRTGQYLLNKDDVLTRVLEVVKNFEKVDASKVTPQSHFVNDLGLNSLDVVEVVFAIEQEFILDIPDHDAEKIQSITDAVEYISQNPMAK;> MSVPSAIRIDTRVAYRRLIKVADQVTRDCPLYQTEGLRQY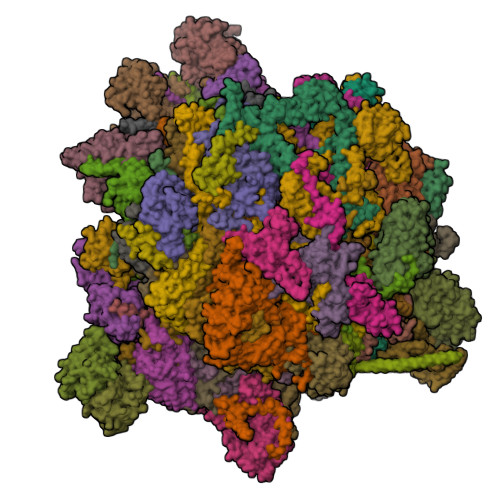VGRRFLERAERNRQQYRHLLHDGSGDARGGRRKFQKQRVLTAQYGKFIAKELQQVHGLAELLLRAPGNTALTSMLQVLSAGVGNVHYQQTVERNYVRYCQFEEKKLDRDEVEEEATSDRQNRIMQHALIPYGERLLILHRLQETGGGRDAVAEPGRLTSWQVTEAIVGTRSGVTAHHMSHGKENVVVEVDETFNKQIVYVRCETYDWSRDVERVEIAEAEELRGTVFHAEYLSVALRLCDALMVETPLHAYRSTVLVGHGVGGAVAFCLALLLHARGFDVKNCVTLGAPKCIQKSLARYVHAVNPIRVVLEGDPLIELPVTGAEGDPFVHCGEILLMDNRARADLGSEADMKTREAGRQSEGGRNESTEDLFTAESLSDSLDPSEEPAMGNEEGCVATGDNNDEGDVGGEDLLEQLRLAAKRYSEGFLVNHYVEHLTDTTVRLTYAEGDEVWDEGDYAQMKREDQLGHSFSGSQKWQDELRSPV;> MAFRRLVKRHKITNNQMLLMRRREPYKPTMKDRQEIADRAKLEEFERKNADGLMFVPEKALPPWQKSLAHNAKALGSRINFRGFRVRVADGQDEPGFPTPFR In order to identify novel CARF effectors, we used Foldseek18 to search for proteins with structural homology to CARF domain of the Cam1 effector. This method rendered a 600-residue protein containing an N-terminal CARF domain followed by a linker region and a C-terminal adenosine deaminase (ADA) domain, with accession number HAJ98955.1 from an unknown Bacteriodales bacterium (hereafter named CRISPR-associated deaminase, CRISPR-associated adenosine deaminase 1 [Cad1]), for which homologs were already identified in a previous bioinformatic screen. cad1 is located immediately downstream the cas10-csm genes of a type III-A CRISPR locus. Further analysis of cad1 homologs showed that over 70% associate in genomes containing type III systems (mostly belonging to the A and B subtypes) and exist within many unique phyla of bacteria. These data suggest that Cad1 is a widespread effector in type III CRISPR-Cas systems. Altogether, these data demonstrate that Cad1 deaminates ATP molecules to ITP through the formation of an hexameric complex that requires a Mg+2 or Mn+2 cofactor and an activating cA4 or cA6 ligand. While the triggering of a growth arrest in the host is a common strategy of all CARF effectors, we believe that Cad1 introduces a new mode of defense for CRISPR-Cas systems that couples nucleotide deamination activity to a sequence-specific, RNA-guided adaptive immune response.

Given that ATP is the putative substrate of Cad1, we obtained cryo-EM structures in the presence of this molecule and found two different conformations with either symmetric (3.4 Å resolution) or asymmetric (3.6 Å resolution) positioning of three ATPs. In both cases, one ATP molecule was bound per Cad1 dimer, unexpectedly not in the deaminase domain (inset with red border) but within a closed (not the open) inter-domain pocket lined with amino acid side chains belonging to both the CARF and ADA domains. We wondered whether this mode of ATP binding was important for Cad1 activity, and therefore, we mutated the basic residues shown to interact with this molecule in the solved structures (inset). In all cases, we made aspartate substitutions to change the charge of these residues and found that while K584D, R588D, K164D, and R162D did not affect Cad1 activation in staphylococci, K589D (within the deaminase domain), R161D, and K165D (within the CARF domain) prevented a complete growth arrest. Third, we unexpectedly found ATPs bound in inter-domain pockets between the CARF and deaminase domains, with three ATPs (anti-glycosidic bonds) in apo-Cad1 hexamer increasing to six ATPs (syn-glycosidic bonds) in the ligand-containing complex. This observation suggests that ATP binding to non-deaminase inter-domain pockets impacts the activation of the deaminase active site. The structures of individual ATP-bound Cad1 dimers (in a hexameric context) in the absence and presence of cA4 did not exhibit major conformational changes between states.

>[6x]MSRVLLCSAGHSSMVVPEAFHAVPEGFEEVHVFTTDSEKFNPVVLNDFFHSLPNVRFSITKCHGLADILNERDFEFYQEMLWQWYLTKMPDNELPYVCLSGGIKSMSASLQKAATLFGAQSVFHVLADNNPRNIEEMFDALQKGQIHFIEMGYEPGWAALRRLKKILPINEGCSRDNFKPLISKSIEEILSNVKIMASDTGKSNQLPFPSLAILPPIAQQWLQLPLSANDGAWIQNLPKVDLHCHLGGFATSGSLLDQVRGAASEPDLIDRTFSPQEIAGWPRSHKSISLDKYMELGNANGSKLLKDKGCLIRQVELLYQSLVNDNVAYAEIRCSPNNYADKNKNRSAWVVLQDINDTFTRLITEAKQKNQFYCHVNLLVIASRKFSGDLSDISKHLALAITAMQQGEGVCRIVGVDLAGFENKETRASYYEHDFKAVHRCGLAVTAHAGENDDPEGIWQAVYSLHARRLGHALNLLEAPDLMRTVIERKIGVEMCPYANYQIKGFAPMPNFSALYPLKKYLEAGILVSVNTDNIGISGANLSENLLILADLCPGISRMDVLTIIRNSIETAFISHDFRMELLKFFDRKIYDVCLISIKN> ASSSSKSSDSSAPKAYGYVYTADPETLDYLISSKNSTTVVTSNGIDGLFTNDNYGNLAPAVAEDWEVSKDGLTYTYKIRKGVKWFTSDGEEYAEVTAKDFVNGLKHAADKKSEAMYLAENSVKGLADYLSGTSTDFSTVGVKAVDDYTLQYTLNQPEPFWNSKLTYSIFWPLNEEFETSKGSDFAKPTDPTSLLYNGPFLLKGLTAKSSVEFVKNEQYWDKEN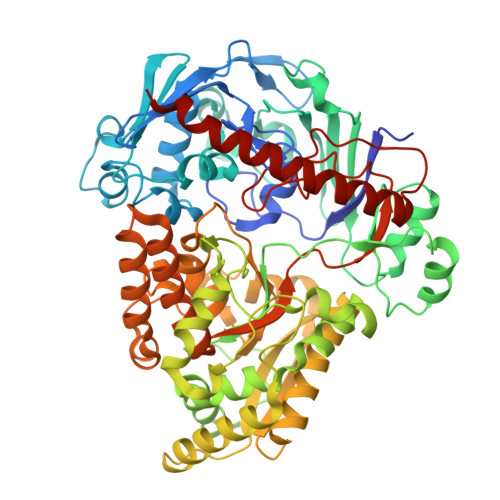VHLDTINLAYYDGSDQESLERNFTSGAYSYARLYPTSSNYSKVAEEYKDNIYYTQSGSGIAGLGVNIDRQSYNYTSKTTDSEKVATKKALLNKDFRQALNFALDRSAYSAQINGKDGAALAVRNLFVKPDFVSAGEKTFGDLVAAQLPAYGDEWKGVNLADGQDGLFNADKAKAEFAKAKKALEADGVQFPIHLDVPVDQASKNYISRIQSFKQSVETVLGVENVVVDIQQMTSDEFLNITYYAANASSEDWDVSGGVSWGPDYQDPSTYLDILKTTSSETTKTYLGFDNPNSPSVVQVGLKEYDKLVDEAARETSDLNVRYEKYAAAQAWLTDSSLFIPAMASSGAAPVLSRIVPFTGASAQTGSKGSDVYFKYLKSQDKVVTKEEYEKAREKWLKEKAESNEKAQKELASHVK To parasitize a phage, the SaPIs employ a transcriptional repressor, Stl, which in addition to repressing the SaPI genes, senses an active phage infection by binding to the phage-encoded anti-repressor protein. Here, we show that the phage satellite SaPI2, which does not encode orthodox anti-phage defense systems, provides antiviral immunity mediated by Stl2, the SaPI2-encoded transcriptional repressor. Stl2 targets and inhibits phage-encoded HRs, including Sak and Sak4, two HRs from the Rad52-like and Rad51-like superfamilies. Here we have focused on two recombinases, an annealase called Sak, and a recombinase called Sak4, belonging to the Rad52-like and Rad51-like superfamilies respectively.

The most abundant particles revealed an architectural structure formed by fifteen Stl2 dimers acting as a molecular filigree decorating two heptadecameric Sak80α rings, keeping them apart and generating a ~ 1.5 MDa structure. As a result of the asymmetry between the number of Sak80α and Stl2 protomers, two Sak80α subunits in each ring were missing any CTD density while a further two had at least partial albeit extremely poor-quality densities, which were left unmodelled. The structure instantaneously elucidates how Stl2 is inhibiting Sak80α by interacting with and corsetting Sak80α’s CTD. To our knowledge, this is the first visualization of the α-helical bundle present in the CTD of a full-length Rad52-like annealase. An overlay of Sak80α models revealed that the CTD was fixed in two different conformations, either up or down, which in relation to Sak80α’s ssDBG might be seen as open (up) or closed (down). This flexibility in Sak80α, provided by the loop connecting α-helices 4 and 5, is suggestive of Sak80α’s mechanism to load ssDNA onto its ssDBG (see discussion). Despite the modest resolution of this region of the map, it could be perceived that Stl2 employs its two loops in the CTD to interact and fix one Sak80α CTD. Mass photometry analysis of Stl2-Loop 1 mixed with Sak80α revealed the formation of larger peaks corresponding to 1 and 1.5 MDa similar to the wild-type, while mixing Stl2-Loop 2 with Sak80α did not generate such peaks, thus indicating that the residues mutated in Stl2-Loop 2 were critical for complex formation. When Stl2 is present, two Sak80α rings are ensconced within a Stl2 armor, preventing Sak80α’s CTD from engaging with anything beyond the Stl2 cage. The two Sak80α rings are kept separated so that they cannot interact to each other, a proposed intermediate step for efficient complementary ssDNA annealing.

>TEQTLFEQLNSKNVNDHTEQKNGLTYLAWSYAHQELKKIDPNYTVKVHEFPHPDINTENYFVPYLATPEGYFVQVSVTVKDSTETEWLPVLDFRNKSLAKGSATTFDINKAQKRCFVKASALHGLGLYIYNGEELPSASDNDITELEERINQFVNLSQEKGRDATIDKTMRWLKISNINKLSQKQIAEAHQKLDAGLKQLDSEEKQ[34x];>MGIRNRLSELLSERGLKISRVAKDVKIARSSLTSMAQNDSEMIRYDAIDKLCSYLHISPSEFFEHNPINFDFTFDEEPNYKINDVFEGFEVTANITHAFSIENFDFEILVDVELDNRQKLNFDLDVSYKETEKITNSQHRFIFTIKNEDENIGLKKYVDSLSAGLKNLLFKKINQKLSGYVSEIIVKNIDDIEELFPNKGEKSTTLHKEILQTDSRLSSDIFKEYGSHHHHHH[30x]WD40 proteins are a subfamily of propeller proteins with no intrinsic enzymatic activity, but their stable, modular architecture and versatile surface have allowed evolution to adapt them to many vital roles. By computationally reverse-engineering the duplication, fusion and diversification events in the evolutionary history of a WD40 protein, a perfectly symmetrical homologue called Tako8 was made. A different computational approach was employed to redesign Tako8 to create Ika8, a fourfold-symmetrical protein in which neighbouring blades carry compensating charges. Tako and Ika are the first successfully designed eight-bladed WD40-repeat proteins for which structures have been confirmed crystallographically.

The concentration of negatively charged residues reflects their high conservation in the parental template structures, so Ika8 was designed as a fourfold-symmetrical protein, allowing the search algorithm to identify compensating interactions between adjacent blades. Ika8 produced two crystal forms in space group P63, with one or three copies in the asymmetric unit. In one crystal form of Ika8 this axis is crystallographic, but in the other (and in the Ika4 crystals) it is noncrystallographic. In all crystal forms, the Ika proteins assemble as trimers which stack on top of each other into pillars. Unlike in the Tako8 protein, the conserved inter­actions stabilizing the crystal assembly involve hydrogen bonds between the outer rims of neighbouring molecules, while the interactions at the top face are mediated by water molecules and are not conserved. In comparison, only the alternating repeats of the Ika proteins can be superposed, in contrast to the template structure where the overlap of the individual blades is much poorer. The symmetry is also visible in the electrostatic potential map, where eightfold and fourfold symmetry can be observed for Tako8 and Ika8, respectively, with the exception of small differences owing to crystal-packing inter­actions; such charge symmetry is absent from the template protein. The melting/denaturation curves show that the Ika proteins are more stable than Tako8, especially under low-salt conditions.

>[3x]GSHMGQELVSLEGHQSAITALAFSKNIVVSGAADGTIKVWDILTGQLLRDHDGHQSEVTALQFKDNIVVSGAKDGTVKVWYIGTGQELVSLEGHQSAITALAFSKNIVVSGAADGTIKVWDILTGQLLRDHDGHQSEVTALQFKDNIVVSGAKDGTVKVWYIGTGQELVSLEGHQSAITALAFSKNIVVSGAADGTIKVWDILTGQLLRDHDGHQSEVTALQFKDNIVVSGAKDGTVKVWYIGTGQELVSLEGHQSAITALAFSKNIVVSGAADGTIKVWDILTGQLLRDHDGHQSEVTALQFKDNIVVSGAKDGTVKVWYIGT> MNDRIIPRNSLYDVATFKLLSDGKDITNDYTVLSITVNQIVNRVPTARIILRDGAAADETFAASEGADLVPGQEVEIAAGYDGSDQKIFQGLIVKHALKVTANGDSMLMLDCRGLATKLTVGRHNRYFVDTKDSDAIAEIIAQHSLSADVAATQVQHPEIVQYYATDWDFILSRAEMNGQIVVAQD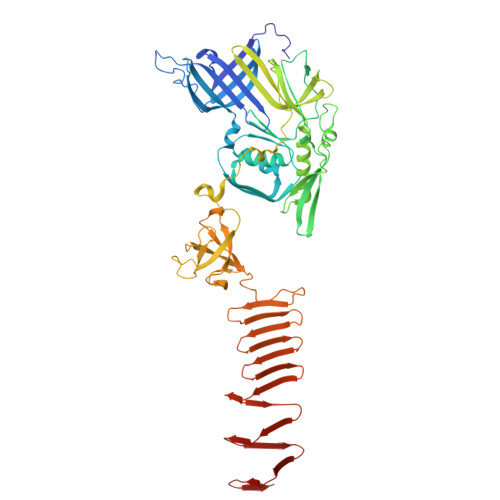EKIKVKAPNTSGAPQITLTYGVNLLELEAAMDARHQYQAVKATSWNYADQALVEAEASEPTVNNQGNLSGRQLAQVIDLSALELRHSGLVAEPELKAWADAQLLKSRLAKIQGRVKTKGYPDAKVDVLIQLAGVGDRFNGLAYVSGIRHEIVGGAWDTHIQMGLPPQWFYQEVDIIDKPAAGLLPGVNGLQIGVVVQLQDDPNGEDRILVKVPIIDAQAEGIWARIATLDAGNNRGSFFRPEVGDEVILGFLNDDPRDPVVLGMLNSSAKPAPLRATAENHRKGFFTRSQMQLTFDDDKKIITLQTPGGNKVTISDEDKGITLTDQNGNTFAMSDRGIAMNSPKDITLEATGKLTLKATQDVSIEGLNVNIAANAQFKAQGNAGAEVSSSAIAVLKGSLVMIN> ADPFTLQPAAHTGAARSCRFRGRHYKREFRLEGEPVALRCPQVPYWLWASVSPRINLTWHKNDSARTVPGEEETRMWAQDGALWLLPALQEDSGTYVCTTRNASYCDKMSIELRVFENTDAFLPFISYPQILTLSTSGVLVCPDLSEFTRDKTDVKIQWYKDSLLLDKDNEKFLSVRGTTHLLVHDVALEDAGYYRCVLTFAHEGQQYNITRSIELRIKKKKEETIPVIISPLKTISASLGSRLTIPCKVFLGTGTPLTTMLWWTANDTHIESAY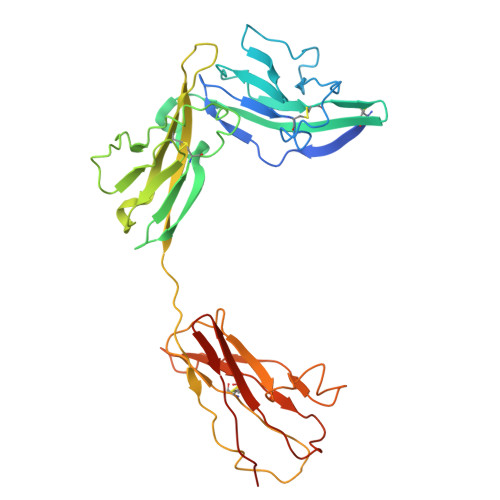PGGRVTEGPRQEYSENNENYIEVPLIFDPVTREDLHMDFKCVVHNTLSFQTLRTTVKEHHHHHH>[4x]GMGSSRKVIITCAVTGAIHTPSMSPYLPVTPDEVAQASIGAAEAGAAVIHLHARDPRDGRPTQDPAAFAEFLPRIKSNTDAVINLTTGGSPHMTVEERLRPATHYMPELASLNMGSMNFGLYPMLERFKEFAHGWEREHLERSRDLVFKNTFADIEFILKTCGGNGTRFEFECYDTSHLYNLAHFVDRKLATPPFFVQTVF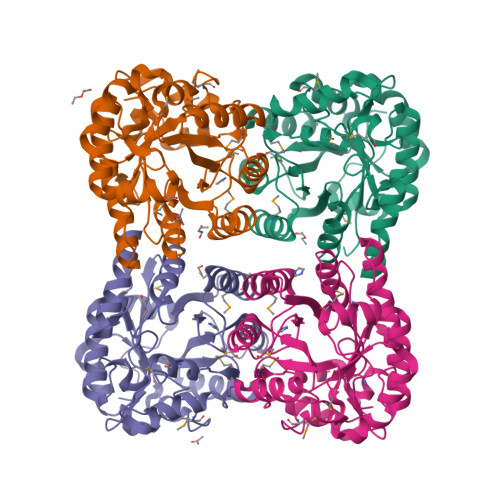GLLGGIGPHPEDLAHMRRTADRLFGADYVWSILGAGRHQIPLASIGAAQGANVRVGLEDSLWIAPGELAETNAAQVRKIRQVIEGLSLEVASPAEARTMLGLKGPQNVNF3-(4-AMINO-1-TERT-BUTYL-1H-PYRAZOLO[3,4-D]PYRIMIDIN-3-YL)PHENOL | C15 H17 N5 O | 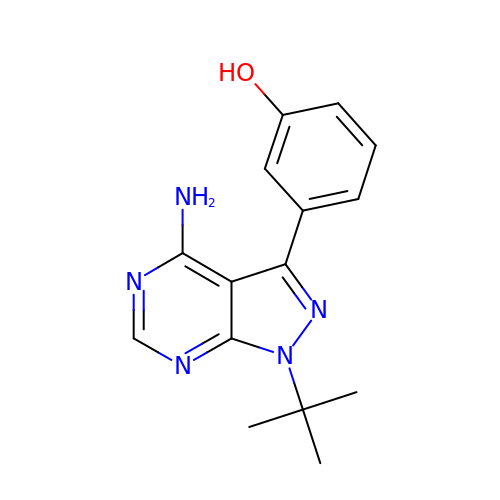CPLGZXQPPYRNRC-UHFFFAOYSA-N To protect viral DNA against the host bacterial restriction system, bacterio­phages utilize a special modification system – hydroxymethylation – in which dCMP hydroxymethylase (dCH) converts dCMP to 5-hydroxymethyl-dCMP (5hm-dCMP) using N5,N10-methylenetetrahydrofolate as a cofactor. Despite shared similarity with thymidylate synthase (TS), dCH catalyzes hydroxylation through an exocyclic methylene intermediate during the last step, which is different from the hydride transfer that occurs with TS. The dCH from T4 bacteriophage (T4dCH) was the first identified viral enzyme, which catalyzes the conversion of dCMP to 5hm-dCMP using mTHF and water as methyl and hydroxyl donors, respectively. Despite its low sequence identity, dCH belongs to the thymidylate synthase (TS) superfamily due to its similar tertiary structure.

Here, we report the crystal structure of the ternary complex of T4dCH (C148S/D179N mutant) bound to dCMP and THF at 1.9 Å resolution. A reasonable electron density for THF could not be obtained from crystals of T4dCH WT; therefore, the active-site double mutant C148S/D179N was used for crystallization. The THF molecule resides in a narrow and deep binding pocket formed by α-helices B, C and G. The enzymatically active cavity for hydroxymethylation is formed along to the narrow binding site of THF, which links to the dCMP binding site. The THF completely occludes the dCMP molecule from the bulk solvent [Fig. 1(c)]. The Cα root-mean-square deviation (RMSD) between the ternary and binary complex structures is only 0.26 Å, and that between the ternary complex and the apo structure is 0.39 Å. These results suggest that no global conformational changes are triggered by THF binding [Fig. 1(d)]. The closed conformation of the apo or binary complex blocks the PABA ring-binding region. THF binding induces local structural changes in Ile81 and Phe174 [Figs. S5(d) and S5(e)]. The branched side chain of Ile81 and the aromatic ring of Phe174 rotate to the outside of the active site, which opens the PABA ring binding site and simultaneously closes the dCMP binding pocket. In summary, despite the lack of a C-terminal tail, T4dCH also recognizes the same cofactor, THF, using different residues in the THF binding pocket. The main-chain nitrogen and side-chain hydroxyl oxygen of Ser94 form a polar interaction with the side-chain carboxylate of Asp145. Furthermore, a potential key water molecule (Wat1) is located within hydrogen-bonding distance of the carboxylate of Asp145 as well as the N1 atom of the pterin ring [Fig. 3(c)].

> MISDSMTVEEIRLHLGLALKEKDFVVDKTGVKTIEIIGASFVADEPFIFGALNDEYIQRELEWYKSKSLFVKDIPGETPKIWQQVASSKGEINSNYGWAIWSEDNYAQYDMCLAELGQNPDSRRGIMIYTRPSMQFDYNKDGMSDFMSTNTVQYLIRDKKINAVVNMRSNDVVFGFRNNYAWQKYVLDKLVSDLNAGDSTRQYKAGSIIWNVGSLHVYSRHFYLVDHWWKTGETHISKKDYVGKYA>[14x]MVEYTNTFKVAAVQAQPVWFDAAKTVDKTVSNIAEAARNGCELVAFPEVFIPGYPYHIWVDSPLAGMAKFAVRYHENSLTMDSPHVQRLLDAARDHNIAVVVGISERDGGSLYMTQLIIDADGQLVARRRKLKPTHVERSVYGEGNGSDISVYDMPFARLGALNCWEHFQTLTKYAMYSMHEQVHVASWPGMSLYQPEVPAFGVDAQLTATRMYALEGQTFVVCT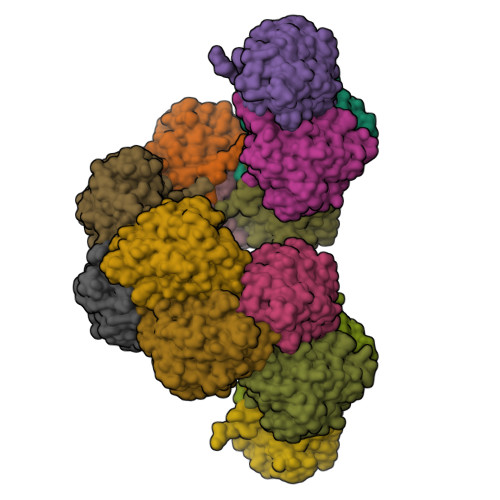TQVVTPEAHEFFCENEEQRKLIGRGGGFARIIGPDGRDLATPLAEDEEGILYADIDLSAITLAKQAADPVGHYSRPDVLSLNFNQRRTTPVNTPLSTIHATH> DFVLDNEGNPLENGGTYYILSDITAFGGIRAAPTGNERCPLTVVQSRNELDKGIGTIISSPYRIRFIAEGHPLSLKFDSFAVIMLCVGIPTEWSVVEDLPEGPAVKIGENKDAMDGWFRLERVSDDEFNNYKLVFCPQQAEDDKCGDIGISIDHDDGTRRLVVSKNKPLVVQF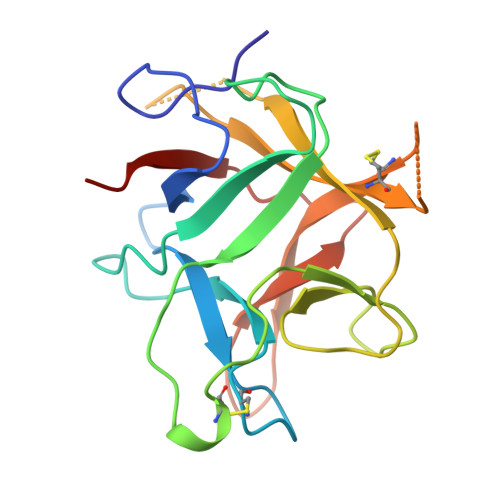QKLDKESL> PQQKRSSPSEGLCPPGHHISEDGRDCISCKYGQDYSTHWNDLLFCLRCTRCDSGEVELSPCTTTRNTVCQ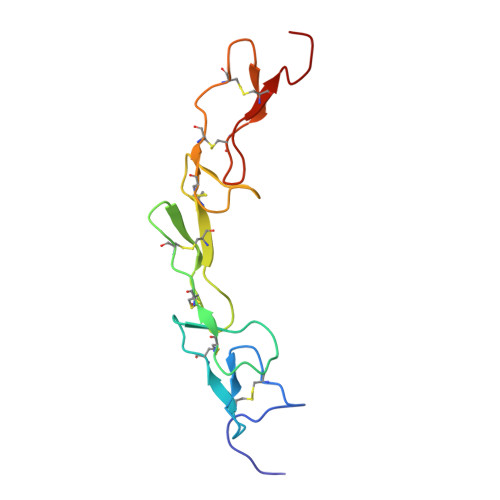CEEGTFREEDSPEMCRKCRTGCPRGMVKVGDCTPWSDIECVHKESGD>[2x]EEVRQFRRLFAQLAGDDMEVSATELMNILNKVVTRHPDLKTDGFGIDTCRSMVAVMDSDTTGKLGFEEFKYLWNNIKRWQAIYKQFDTDRSGTICSSELPGAFEAAGFHLNEHLYNMIIRRYSDESGNMDFDNFISCLVRLDAMFRAFKSLDKDGTGQIQVNIQEWLQLTMYS

Calpain-I and calpain-II are the two most studied members of a family of calcium dependent cysteine proteases that currently comprises fifteen identified gene products in humans. These heterodimeric proteases are composed of a large subunit with a molecular mass of ∼80 000 and a small subunit of mass ∼30 000. Selective inhibitors might not only be potential drugs but should act as tools to explore the physiological and pathophysiological roles of calpain-I. α-Mercaptoacrylic acid based calpain inhibitors are potent, cell permeable and selective inhibitors of calpain-I and calpain-II. These inhibitors target the calcium binding domain PEF(S) of calpain-I and -II.

To test this proposal, the oxidised form of 3, (2Z,2′Z)-2,2′-disulfanediylbis(3-(6-bromoindol-3-yl)acrylic acid), (4), was generated and the single crystal X-ray structure of 4 bound to PEF(S) solved. Compound 4 was then added to preformed crystals of PEF(S). The electron density map revealed that the ligand adopts two different conformations in each subunit of the PEF(S) homodimer, therefore a total of four conformations of the ligand were observed in the asymmetric unit of the crystal structure. The unique geometry of the disulfide bond is observed in all of the conformations ensuring that both pockets of the hydrophobic groove of PEF(S) are explored. One of the 6-bromoindole rings of 4 is bound in the hydrophobic binding pocket that also binds 3. The second indole ring of 4 interacts with a hydrophobic groove on the surface of PEF(S), where the α-helix of CAST inhibitory region C binds with PEF(S). A greater number of interactions form between 4 and residues of PEF(S) than with 3 and the protein, including a number of electrostatic interactions and hydrogen bonds. An electrostatic bond forms between the carboxylate group of 4 and the positively charged guanidinium group of Arg130. The dihedral angle of –91 in chain A is close to the optimum dihedral angle and in this conformation 4 makes strong interactions with both hydrophobic pockets of PEF(S). The restricted geometry of the disulphide bond facilitated a larger number of favourable binding interactions with PEF(S) so that the two aromatic rings of 4 interact with the hydrophobic pockets that bind Leu 660 and Leu 656 of calpastatin.>[4x]MTDFDSLSGTSTTWVNELGSVMTIDVDRKGGVTGYYVNNAPGT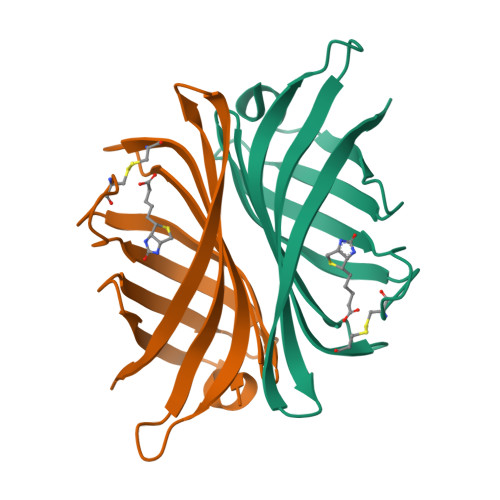GCRGLPYDLSGHAHGSTIAFSVVWSNGIADCRSATSWAGYARKTFGGGVQIVTQWSLAFVGKAGGKIETGQNVFTYQAYDAQPSPADK3-bromophenol | C6 H5 Br O | 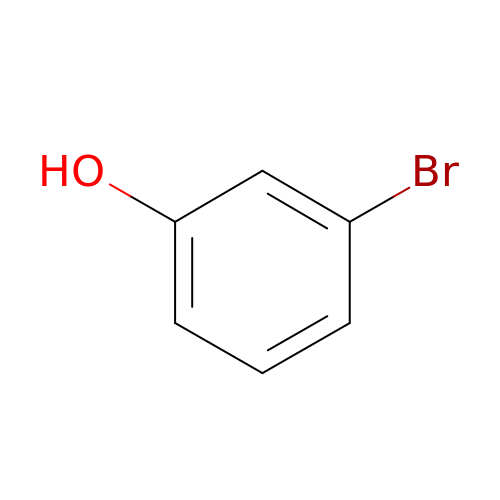MNOJRWOWILAHAV-UHFFFAOYSA-N>GSHMSSVTIGKCYIQNRENGGRAFYNLGRKDLGIFTGKMYDDQIWSFQKSDTPGYYTIGRESKFLQYNGEQVIMSDIEQDTTLWSLEEVPEDKGFYRLLNKVHKAYLDYNGGDLVANKHQTESEKWILFKAY[2x]

SeviL is a recently described lectin, of uncertain biological function, isolated from mussels. Here we have shown the protein is a dimeric member of the well-known β-trefoil superfamily. The β-trefoil fold shows pseudo-three-fold rotational symmetry, with three subdomains of the protein (called α, β and γ) that each contain four β-strands. SeviL is the first lectin to be described that shows an exquisite selectivity for asialo-GM1 over the closely related GM1, suggesting it may well be a useful tool in ganglioside research, and especially in studies of NK cells, which are currently of enormous interest due to their central role in the control of cancer by the immune system.

The two monomers in the dimer are closely associated by hydrophobic interactions and hydrogen bonds involving 11 residues on each subunit. Gln 12 and Phe 126 lie close together, and their side-chains lie opposite their symmetry mates at the dimer interface. Met 36 (and its symmetry mate) contributes the largest contribution of buried surface area of any residue at the interface, becoming entirely sequestered from the bulk solvent. The buried interface area between SeviL monomers is 780 Å2, but too small for PISA28 to predict a stable dimer with confidence. Within the apo crystal structure, a crystal contact is formed with Arg 26 of the B chain approaching within 3.6 Å of its symmetry mate. Two nearby balls of electron density were modelled as chloride ions, which would counter the repulsive charge on the two residues (SFigure 2). One chloride ion sits in a hydrophobic pocket formed by Phe 21, Phe 32 and Tyr 37; it comes within 3 Å of the side-chain of Asp 39, which also lies close to Arg 26 from the neighbouring molecule. No chloride ions were modelled near the A subunit, and it appears this interaction is unique to the crystal form, which was crystallised at pH 3.5. Comparing the main chain atoms of a single subunit, the apo and liganded forms show a rmsd of up to 0.36 Å, depending on which subunits are compared, indicating that the protein shows no movement on ligand binding. Least-squares comparison of the dimer in the apo and liganded models gives a rmsd of 121 Cα atoms (residues 9–129) of 0.53 Å.> MAAQHGAPPSARSPRFGVNYTPSNGWFHHWLDFDLDAVRADLDSVAALGFDHVRVFPLWPVFQPNRTLIRPRAVEQLAALTDAAGERGLDVNVDGLQGHLSSF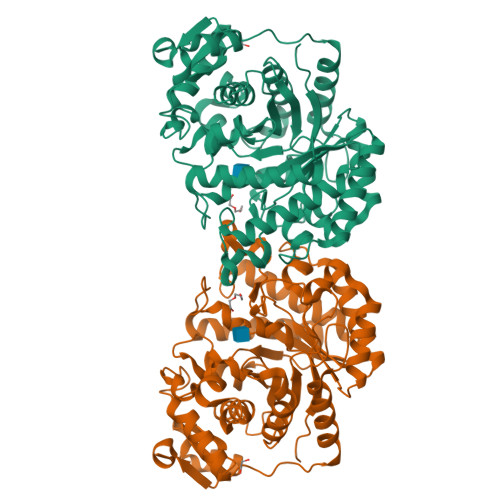DFLPAWTTTWHRRNLFTDPDVVSGQAEYLRTLAAALADRPNFLGMTVGNEINQFSGHPHPDPDRVTPEQAGDWLRRMLDACERGAPGRLHLHAEYDAAWYLDDHPFTPAHSARIGAVTAVHSWVFNGTAQRYGTRSTATAQHAAYLVELAKAWAREPRRPVWLQEVGAPAPHVPAEYAAEFATATIDAVLDCPEVWGVTWWCSHDVDRRLADFPELEYSLGLLTQDRRVKPAGRAVAEAVRRWRTETPAPRPRTTALVVDVGPGDQAPARSVCAPGGAVFEAFMRLTAQGARPTTVLAEHATDADHLAARGITEVVTPHDVHLEHHHHHH TcXyn30B is a bifunctional xylanase with endo‐glucuronoxylanase and exo‐xylobiohydrolase activities. The present study provides insight into the mechanisms of substrate recognition of a bifunctional xylanase.

The present study determined the crystal structure of the TcXyn30B‐product complex. A 4‐O‐methyl‐α‐d‐glucuronyl moiety‐binding pocket required for glucuronoxylanase activity and Asn‐93 (which is likely involved in xylobiohydrolase activity) was structurally characterized.

> MRFPSIFTAVLFAASSALAAPVNTTTEDETAQIPAEAVIGYSDLEGDFDVAVLPFSNSTNNGLLFINTTIASIAAKEEGVSLEKREAEAYVEFQINVDLQARYQSVDGFGCSQAFQRAEDIFGKYGLSPKNQSYVLDLMYSEERGAGFTILRNGIGSSNSSTSNLMNSIEPFSPGSPSSTPNYTWDHYNSGQFPLSQQARARGLPYIYADAWSAPGYMKTNQDENWSGFLCGIEGETCPSGDWRQAYADYLVQYVKFYAESGVPVTHLGFLNEPQEVVSYASMGSNGTQAAEFVKILGQTLEREGIDIELTCCDGVGWSEQEAMIPGLQVVGPDGKSAEDYLSVVTGHGYSSAPTFPLSTKRRTWLTEWTDLSGAFTPYTFFADGGAGEGMTWANHIQTAFVNANVSAFIYWIGAENSTTNSGMINLINDEVIPSKRFWSMASFSKFVRPNAQRVKATSSDASVTVSAFENTNGVVAIQVINNGTSAASLTIDLGKTHKEVKKVVPWVTSNDYDLEEMSEIDVKHNSFLASVPARSLTSFVTECE> MAHHHHHHESETTTSLVLERSLNRVHLLGRVGQDPVLRQVEGKNPVTIFSLATNEMWRSGDSEVYQLGDVSQKTTWHRISVF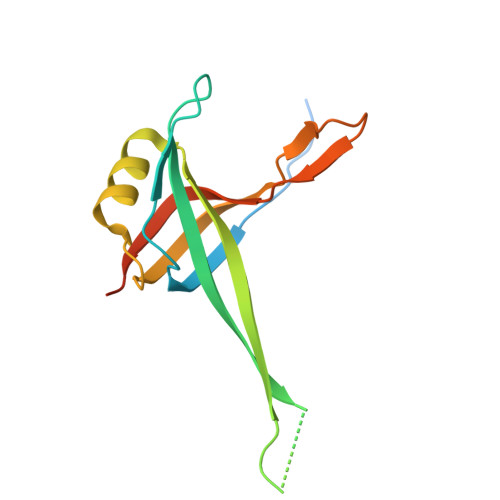RPGLRDVAYQYVKKGSRIYLEGKIDYGEYMDKNNVRRQATTIIADNIIFLSDQTKEKELE> CSEGLEDIDGNPRNITQEQLEVDFQNVGSLYKPMFENIYQYTPPWSYQLQQNLNA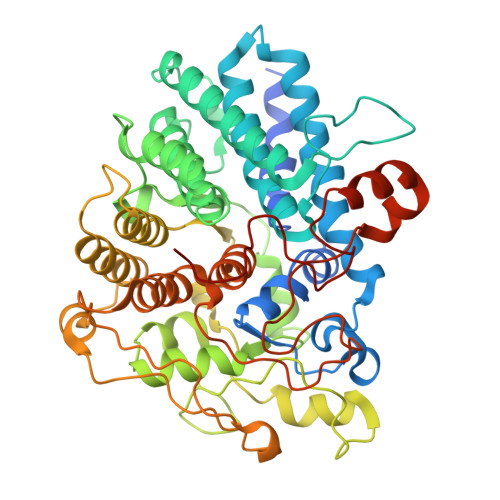DVFSGYMTNPRPFVAGANNTTYNLVSGWNNFIWSVPYSNVMNNAKTIEEETKDEFPELFAVSQILKVTAMHRVADVFGPIVYTKFGESATTSEYDSQEEAYNAFFNDLEEAIQILSDNIDSPRFTAFDLAYGGNYTNWIKYANSLRLRLAIRISKVSPAKAKSEGEKSLNHSLGVIETNPDGFFVNGTLDHPVRTINNSWGDIRMNASMESILVGYEDPRVDSYFNASEVVEGEFKGIRNGLPLLSEYDDELAQKADYITFSLLSDEVLTPRVQLMTAAEVFFLKAEAALRGWSGAGDTRTNYEQGITTSFQQYGLSGISEYIANNTRTPIDYVDPVTPANNINALSTITIEWDEAASNEEKLERIITQKWIALFPEGQEAWSEYRRTGYPKIFPVISNQSGGVVDTDLQIRRIPFVDSELQTNPDGVADAITKLGGPDNAGTRLWWDVPGGNFLEHHHHHH(3,5-difluorophenyl)methanol 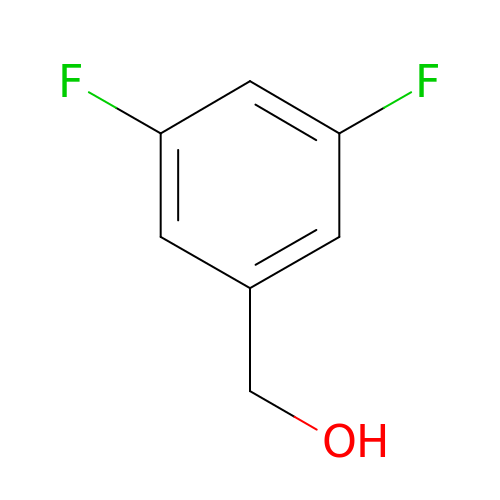| C7 H6 F2 O | LOGIHEKXJKHXEC-UHFFFAOYSA-N>[2x]MKNKVQLITYADRLGDGTIKSMTDILRTRFDGVYDGVHILPFFTPFDGADAGFDPIDHTKVDERLGSWDDVAELSKTHNIMVDAIVNHMSWESKQFQDVLAKGEESEYYPMFLTMSSVFPNGATEEDLAGIYRPRPGLPFTHYKFAGKTRLVWVSFTPQQVDIDTD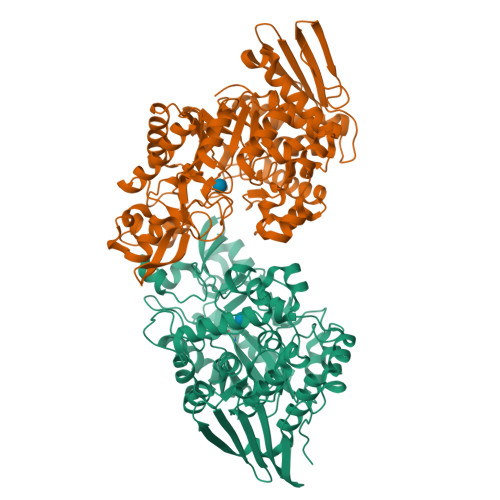SDKGWEYLMSIFDQMAASHVSYIRLDAVGYGAKEAGTSCFMTPKTFKLISRLREEGVKRGLEILIEVHSYYKKQVEIASKVDRVYDFALPPLLLHALSTGHVEPVAHWTDIRPNNAVTVLDTHDGIGVIDIGSDQLDRSLKGLVPDEDVDNLVNTIHANTHGESQAATGAAASNLDLYQVNSTYYSALGCNDQHYIAARAVQFFLPGVPQVYYVGALAGKNDMELLRKTNNGRDINRHYYSTAEIDENLKRPVVKALNALAKFRNELDAFDGTFSYTTDDDTSISFTWRGETSQATLTFEPKRGLGVDNTTPVAMLEWEDSAGDHRSDDLIANPPVVA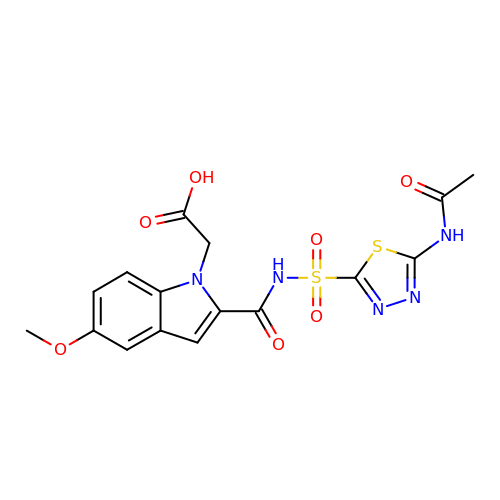[2-({[5-(acetylamino)-1,3,4-thiadiazol-2-yl]sulfonyl}carbamoyl)-5-methoxy-1H-indol-1-yl]acetic acid | C16 H15 N5 O7 S2 | VIHSTBSIMXHLDH-UHFFFAOYSA-N>[4x]MEFTTGLMSLDTALNEMLSRVTPLTAQETLPLVQCFGRILASDVVSP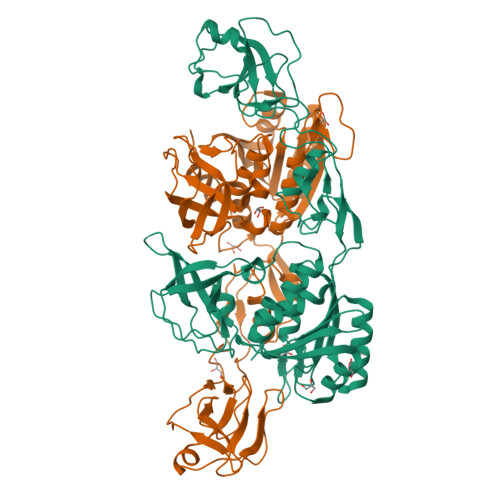LDVPGFDNSAMDGYAVRLADIASGQPLPVAGKSFAGQPYHGEWPAGTCIRIMTGAPVPEGCEAVVMQEQTEQMDNGVRFTAEVRSGQNIQRRGEDISAGAVVFPAGTRLTTAELPVIASLGIAEVPVIRKVRVALFSTGDELQLPGQPLGDGQIYDTNRLAVHLMLEQLGCEVINLGIIRDDPHALRAAFIEADSQADVVISSGGVSVGEADYTKTILEELGEIAFWKLAIKPGKPFAFGKLSNSWFCGLPGNPVSATLTFYQLVQPLLAKLSGNTASGLPARQRVRTASRLKKTPGRLDFQRGVLQRNADGELEVTTTGHQGSHIFSSFSLGNCFIVLERDRGNVEVGEWVEVEPFNALFGGL>GUGUGUAC[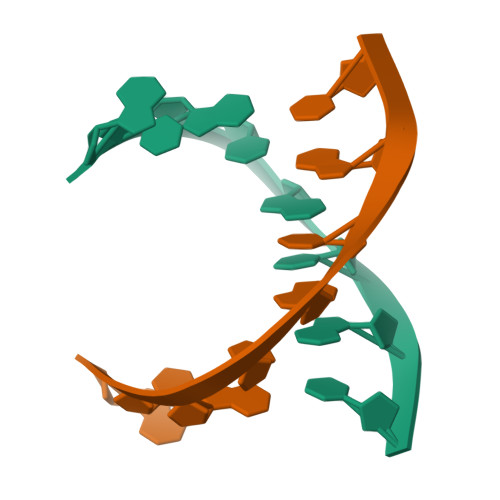2x]> MGAQVSAQKSGTHETGNIATEGSTINFTNINYYKDSYAASASRQDFTQDPTKFTSPVLDAIKEAAAPLQSPSVEACGYSDRVAQLTVGNSTITTQEAANIVLSYGEWPGYCPSTDATAVDKPTRPDVSVNRFYTLSTKSWKTESTGWYWKFPDVLNDTGVFGQNA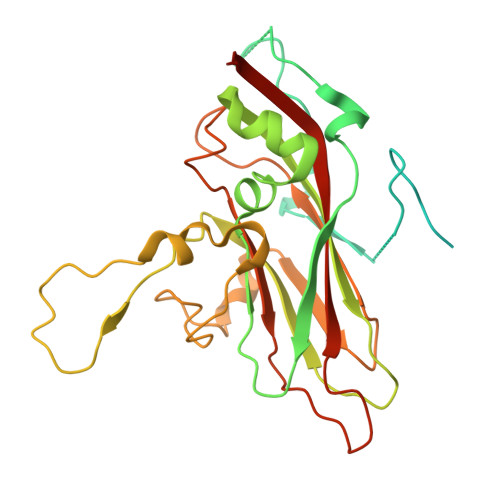QFHYLYRSGFCMHVQCNASKFHQGALLVVVIPEFVVAASSPATKPNGQGLYPDFAHTNPGKEGQVFRDPYVLDAGIPLSQALVFPHQWINLRTNNCATIIMPYVNALPFDSALNHSNFGLAVIPISPLKYCNGATTEVPITLTIAPLNSEFSGLRQAIKQ>HMVKVGYIQMEPKILELDKNYSKAEKLIKEASKEGAKLVVLPELFDTGYNFESREEVFDVAQQIPEGETTTFLMELARELGLYIVAGTAEKSGNYLYNSAVVVGPRGYIGKYRKIHLFYRE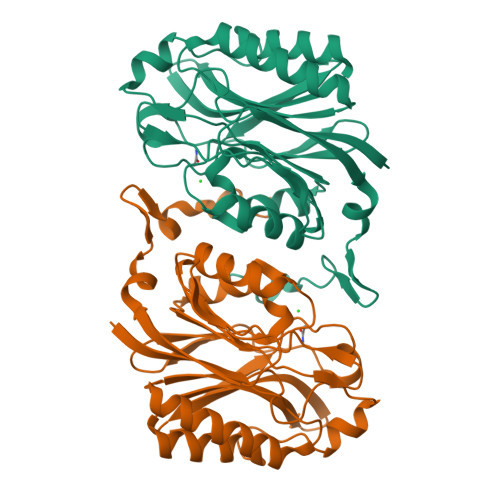KVFFEPGDLGFKVFDIGFAKVGVMIAFDWFFPESARTLALKGAEIIAHPANLVMPYAPRAMPIRALENRVYTITADRVGEERGLKFIGKSLIASPKAEVLSIASETEEEIGVVEIDLNLARNKRLNDMNDIFKDRREEYYFR[2x]>[12x]MQLFDLSLEELKKYKPKKTARPDFSDFWKKSLEELRQVEAEPTLESYDYPVKGVKVYRLTYQSFGHSKIEGFYAVPDQTGPHPALVRFHGYNASYDGGIHDIVNWALHGYATFGMLVRGQGGSEDTSVTPGGHALGWMTKGILSKDTYYYRGVYLDAVRALEVIQSFPEVDEHRIGVIGGAQGGALAIAAAALSDIPKVVVADYPYL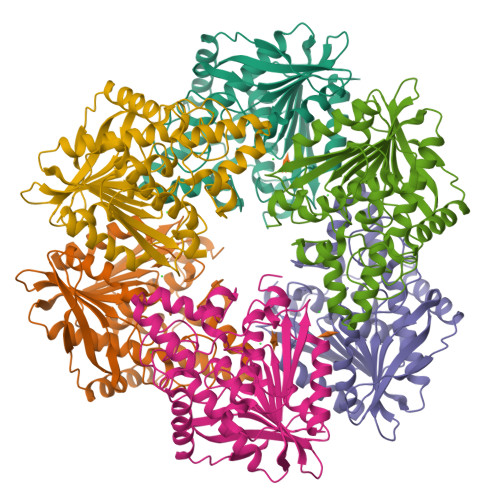SNFERAVDVALEQPYLEINSYFRRNSDPKVEEKAFETLSYFDLINLAGWVKQPTLMAIGLIDKITPPSTVFAAYNHLETDKDLKVYRYFGHEFIPAFQTEKLSFLQKHLLLST>MSFDINWSTLESDNRLNDLIRKHLNSYLQNTQLPSYVSNLRVLDFDLGKVGPAITLKEITDPLDEFYDSIREEADQETEENNDNKEDSEHICPDRTIANHEGPKDDFEAPVVMPSPNDIQFLLEVEYKGDLLVTIGADLVLNYPVEKFMTLPVKLSISDIGLHSLCIVACLSKQLFLSFLCDVSDPALDDN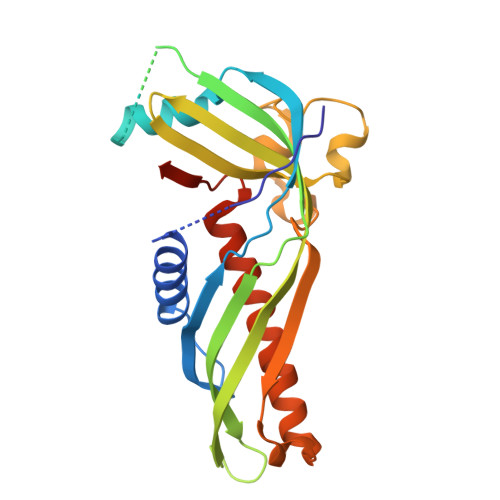QTVLDPKGPILAATKPLERISIVRSMKIETEIGEQYQGQGSVLRSVGELEQFLFTIFKDFLRKELAWPSWINLDFNDGDELVPR[2x]>[2x]ANPYERGPDPTESSIEAVRGPFAV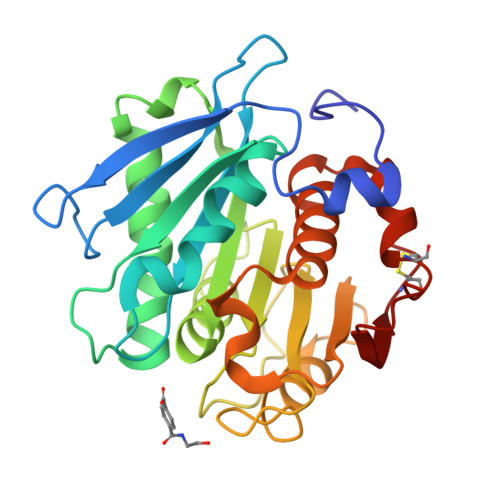AQTTVSRLQADGFGGGTIYYPTDTSQGTFGAVAISPGFTAGQESIAWLGPRIASQGFVVITIDTITRLDQPDSRGRQLQAALDHLRTNSVVRNRIDPNRMAVMGHSMGGGGALSAAANNTSLEAAIPLQGWHTRKNWSSVRTPTLVVGAQLDTIAPVSSHSEAFYNSLPSDLDKAYMELRGASHLVSNTPDTTTAKYSIAWLKRFVDDDLRYEQFLCPAPDDFAISEYRSTCPF> LI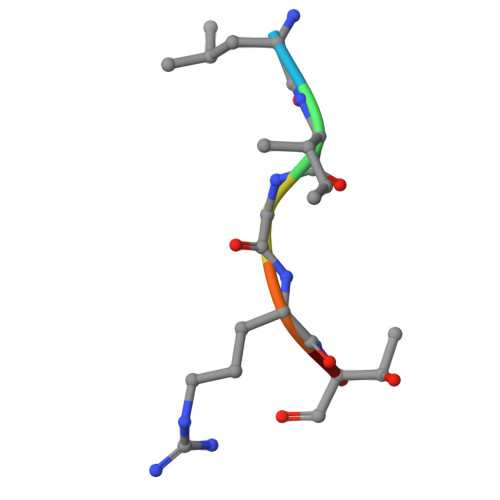GRTQ> DPSDYAEPMDAVV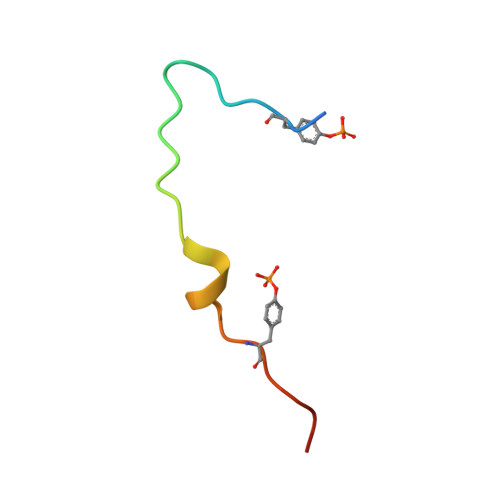KPRNEEENIYSVPHDS alpha-D-xylopyranose | C5 H10 O5 | 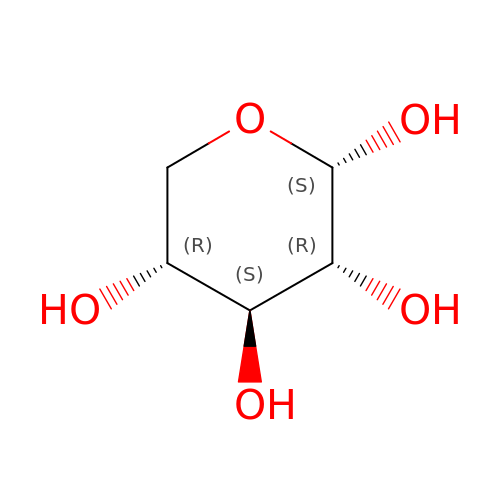SRBFZHDQGSBBOR-LECHCGJUSA-N>[2x]MTSGSLQFTVLRAVNPATDAQRESMLREPGFGKYH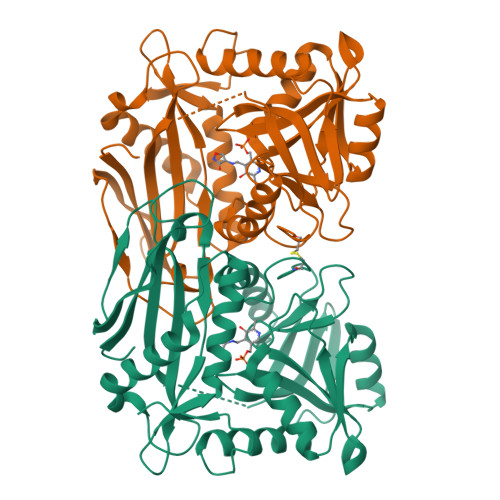TDHMVSIDYAEGRGWHNARVIPYGPIELDPSAIVLHYAQEVFEGLKAYRWADGSIVSFRADANAARLRSSARRLAIPELPDAVFIESLRQLIAVDKAWVPGAGGEEALYLRPFIFATEPGLGVRPATQYRYLLIASPAGAYFKGGIAPVSVWVSTEYVRACPGGTGAAKFGGNYAASLLAQAEAAENGCDQVVWLDAVERRYIEEMGGMNIFFVLGSGGSARLVTPELSGSLLPGITRDSLLQLAIDAGFAVEERRIDIDEWQKKAAAGEITEVFACGTAAVITPVARVRHGASEFRIADGQPGEVTMALRDTLTGIQRGTFADTHGWMARLG>[3x]MQRFN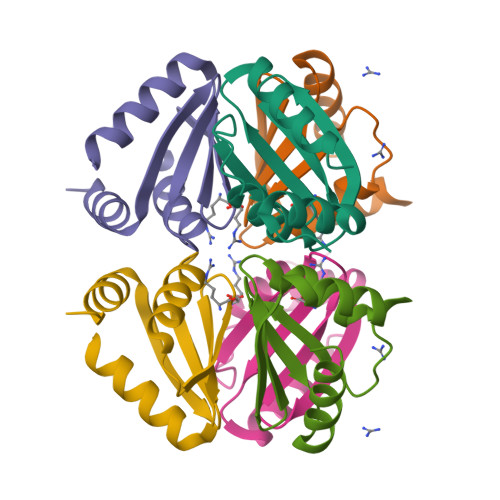PLSKLKRALMDAFVKIDSASHMIVLKTMPGNAQAIGALMDNLDWDEMMGTICGDDTILIICRTPEDTEGVKNRLLELL>MADISRAEVATLIEEGYSHSLLAAAKQGSTVLSAFQNVNMGTKTTHLPVLATLPEADWVGESATDPEGVIKTSKVTWANRTLVAEEVAVIIPVPEAVIDDATVELLTEVAEQGGQAIGKKLDQAVMFGIDKPASWVSPALLKAATDAGQAIAHVSGVANEYDLVGASNKVAEQVALAGWAPDTLLSSLALRYQVANVRDADGNLAFRDGSFLGFNTHFNRNGAWSPESAVAFIADSSRVKIGVRQDITVKFLDQATLGTGDNQINLAERDMVALRLKARFAY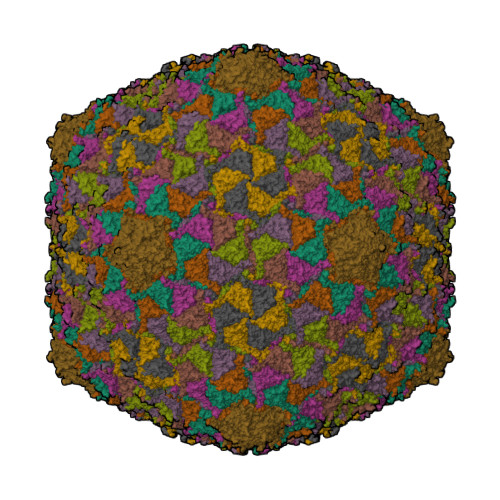VLGVSATAMGANKTPVGVVTPDVTPPTSGE[9x]>[3x]GSMEAVLNELVSVEDLLKFE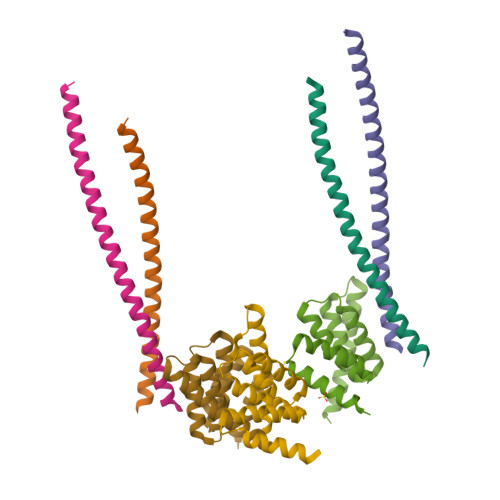KKFQSEKAAGSVSKSTQFEYAWCLVRSKYNDDIRKGIVLLEELLPKGSKEEQRDYVFYLAVGNYRLKEYEKALKYVRGLLQTEPQNNQAKELERLIDKAMKKDGL;>[4x]GSLDVGNAEVKLEEENRSLKADLQKLKDELASTKQKLEKAENQVLAMRKQSEGLTKEYDRLLEEHAKLSAAA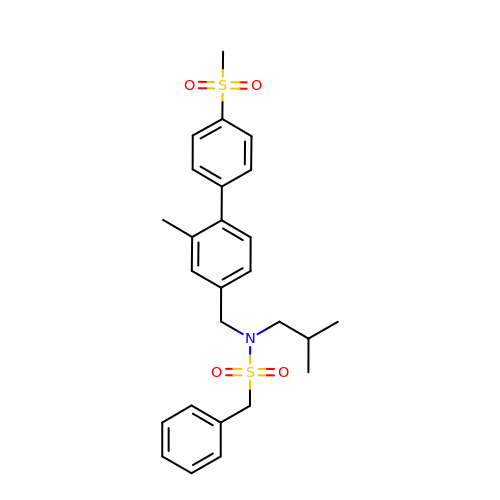~{N}-[[3-methyl-4-(4-methylsulfonylphenyl)phenyl]methyl]-~{N}-(2-methylpropyl)-1-phenyl-methanesulfonamide | C26 H31 N O4 S2 | CMVNZKHEXHXTEM-UHFFFAOYSA-N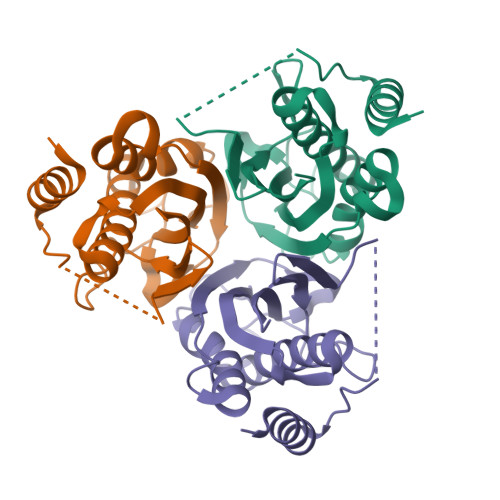>[3x]MNRDDAFLTVQARLGYDFSGDMKIGGKYTSLIEHAGLAYMSGQIPRVEDKVQVCGKVGFDVDLSQAQLAASISTMRALAILKQHYGTLQVVEKVLQMNVFIHSTADFTQQSEVADGASEILYEILGSDTGQHTRTSVSVCQLPKNASVEINFIVALKQNNGQE> MNINEPSGEAANIISQAADSHAMKYYNAADWQAEDNALPSLAELRDLVINQQKSVLFDFSQNSDADGQAEMQAQFRKTYGVGFANQFIFITEHKGELLFTPFEHSEEVDPKLLEAPLTTRSGLKSTAPTNSETSTLPHVAFYISVNRPISDEECTFDNSWLWKDEKGSRPFCKDANISLIYRVNLERSLQYGIVGSATPNAKIVRISLDDDSSGAGIHLNDQLSYRRFGASYTTLDAYFREWSTDAIAQDYRFVFKTSNNKAEILETFPIDNLNVKYEKRKQSGFELGVTGGAEVSEDGPKAKLEARASITQSRWLTYNTQDYRVERNAKNAQTVSFT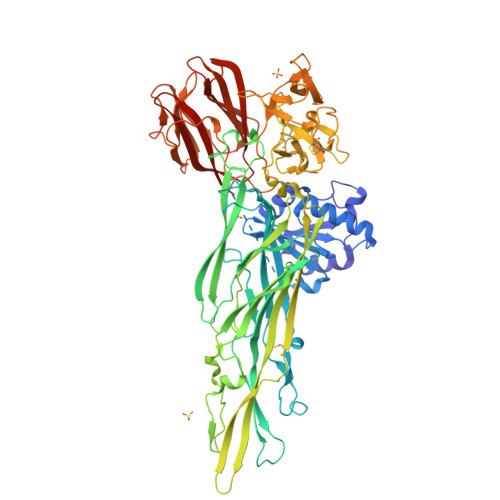WNRQEYATAESLLNRSTDALWVDTYPVDVNRISPLSYASFVPKMDVIYKASDTETGSTDFIIDSSVNIRPIYNGAYKHYYVVGAHQSYHGFENSPRRRITKSASFTVDWDHPVFTGGRPVNLQLASFNNRCVQVDAQSRLTANTCDDQQSAQSFIYDQLGRYVSASNTELCLDGAALDVLQTCNQNLTQRWEWRKNTDELTNVYSGESLGHDKQTGELGLYASSNDAVSLRTITAYTNVFNVQKSSPILGYTQGKMNQQSVGQNYRLYVREGSAIDALGTASDLLVGGNGGSLTSVDLSGVKSITATSGDFQYGGQQLVALTFTYQDGRQQMVGSKAHVTNAHEDRFDLPDAAKITQLNIWADDWLVKGVQFDLNLEHHHHHH>MTSRKKVLLKVIILGDSGVGKTSLMNQYVNKKFSNQYKATIGADFLTKEVMVDDRLVTMQIWDTAGLERFQSLGVAFYRGADCCVLVFDVTAPNTFKTLDSWRDEFLIQASPRDPENFPFVVLGNKIDLENRQVATKR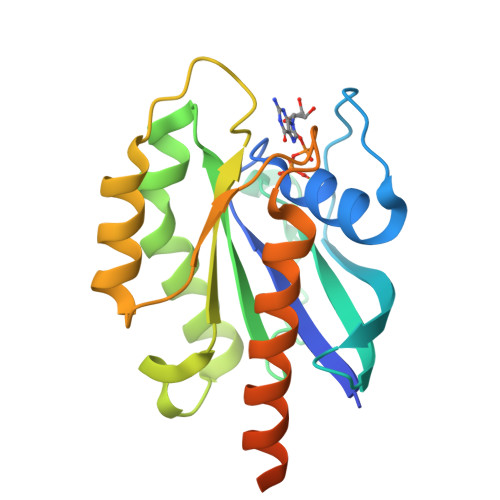AQAWCYSKNNIPYFETSAKEAINVEQAFQTIARNALKQETEVELYNEFPEPIKLDKNDRAKASAESCSC[4x]> AEPSSPPGAPSQPVVTEITKNSITLTWKPNPQTGAAVTSYVIEAFSPAAGNTWRTVADGVQLETHTVSGLQPNTIYLFLVRAVGAWGLSEPSPVSEPVRTQDSSPSRPVEDPWR;> AGYDFCSERHNCMENSICRNLNDRAVCSCRDGFRALREDNAYCEDIDECAEGRHYCRENTMCVNTPGSFMCICKTGYIRIDDYSCTEHDECITNQHNCDENALCFNTVGGHNCVCKPGYTGNGTTCKAFCKDGCRNGGACIAANVCACPQGFTGPSCETDIDECSDGFVQCDSRANCINLPGWYHCECRDGYHDNGMFSPSGESCEDIDECGTGRHSCANDTICFNLDGGYDCRCPHGKNCTGHHHHHH

Robo family receptors are type I transmembrane proteins that instruct neuronal wiring in various organisms, including worms, flies, mice, and humans, in addition to fulfilling diverse functions outside the nervous system. While Robo1 and Robo2 function as classical Slit receptors, the divergent family member Robo3 does not bind Slits and instead acts as a negative regulator of Robo1/2-mediated Slit repulsion. Further, a recently identified Robo3 ligand, NELL2, signals axon repulsion. NELL2 is a secreted glycoprotein containing a laminin G-like (LamG) domain, a coiled coil (CC) domain, and six epidermal growth factor-like (EGF) domains, flanked by five von Willebrand factor type C (VWC) domains.

We next set out to determine the structure of NELL2 in complex with Robo3. Using constructs that include the hNELL2 EGF domains 1–6 and the hRobo3 FN domains 1–3, we obtained a stable complex of these molecules, as demonstrated by size-exclusion chromatography (SEC). Surface plasmon resonance (SPR) analysis of this complex yielded a dissociation constant of 0.6 µM. The NELL2–Robo3 complex structure was determined by an MR-SAD phasing strategy to 2.76-Å resolution. The structure shows direct binding between the NELL2 EGF2 and EGF3 domains and the Robo3 FN1 domain, consistent with our domain mapping data. The two EGF domains wrap around the FN domain and interact with the β-sheet composed of the CDFG strands. To our knowledge, this mode of interaction between EGF and FN domains has not been observed before. The human NELL2–Robo3 complex structure displays a surprising partitioning of the overall binding interface into a highly polar interface at the EGF2–FN1 contact, and an entirely hydrophobic interface at the EGF3–FN1 contact. Several mutations nearly abolish binding, while many others yield diminished binding activities, confirming the validity of the crystallographic model. Thus, the affinity of the NELL2–Robo3 interaction determines NELL2 axon guidance activity.>[4x]SSGIHVA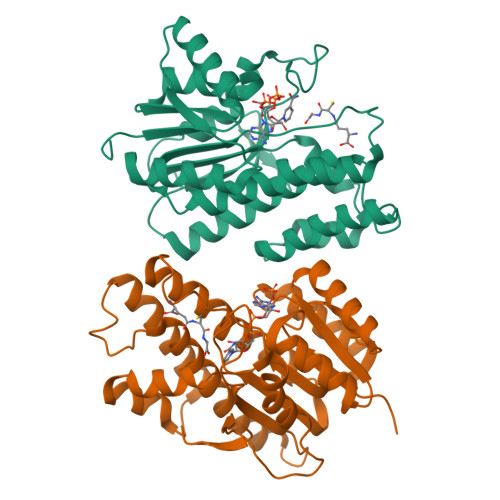LVTGGNKGIGLAIVRDLCRLFSGDVVLTARDVTRGQAAVQQLQAEGLSPRFHQLDIDDLQSIRALRDFLRKEYGGLDVLVNNAGIAFKVADPTPFHIQAEVTMKTNFFGTRDVCTELLPLIKPQGRVVNVSSIMSVRALKSCSPELQQKFRSETITEEELVGLMNKFVEDTKKGVHQKEGWPSSAYGVTKIGVTVLSRIHARKLSEQRKGDKILLNACCPGWVRTDMAGPKATKSPEEGAETPVYLALLPPDAEGPHGQFVSEKRVEQW> LPAPQNLSVLSTNMKHLLMWSPVIAPGETVYYSVEYQGEYESLYTSHIWIPS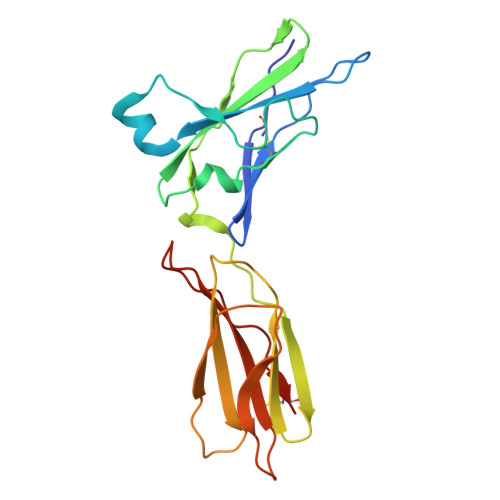SWCSLTEGPECDVTDDITATVPYNLRVRATLGSQTSAWSILKHPFNRQSTILTRPGMEITKDGFHLVIELEDLGPQFEFLVAYWRREPGAEEHVKMVRSGGIPVHLETMEPGAAYCVKAETFVKAIGRYSAFSQTECV>[2x]MTYQWLIGIQISLLFVNCICNGSEWSYTNILTGPETWHEHYKNMCSGYYQSPIDLKTDISTLDLKLKTVIIYRNTSSTETTTIQNNGHSAEVKFPRNTWFISFDGILDYKYEIIQMHFHWGNTDDRGSEHTIDGFRFPLEGHIVSFRRQMYSSPSEAIGRPGGLAVLGIMHQIVESIKYEQTAFKAYNNFSGVLNS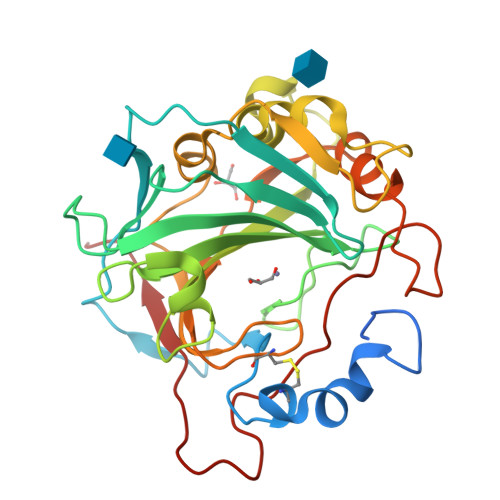QFVPPNNSTIDDINLALLLSLLNPSRYFRYLGSLTTPPCTENVLWTVFIDPVLITREQINLFRNLPYGSNEKQTRMGDNFRPIQLLNPIDTLASRTLYRATARG PMT-based O-mannosylation is an evolutionarily conserved and vital process, key for cell wall integrity and protein quality control in fungi. PMTs are divided into three subfamilies (PMT1, PMT2, and PMT4) and form functional dimers either within or across subfamilies (Akasaka-Manya et al., 2006; Girrbach and Strahl, 2003). In these structures each subunit has 11 transmembrane helices (TMHs) and two large hydrophilic loops oriented towards the ER lumen (LL): loop LL1 between TMH1 and 2 harboring a catalytic DE motif, and loop LL4 between TMH7 and 8, encompassing a so-called MIR domain, whose function remains unknown. MIR domains have a β-trefoil fold consisting of six β-hairpins arranged within a pseudo-threefold symmetry.

The high resolution of the Pmt2-MIR (1.6 Å) and Pmt3-MIR (1.9 Å) structures allowed for a detailed analysis of the respective structural properties and ligand interactions. Amino acid ranges for Pmt2-MIR are 339–401 (MIRm1), 402–466 (MIRm2) and 467–532 (MIRm3). In order to understand the role of PMT-MIR domains in protein O-mannosylation, we analyzed the Pmt2-MIR structure for specific surface properties. On the protein surface two regions reveal high sequence conservation, in the following denoted as sites α and β (residue ranges see Figure 2) in accordance with general CBM terminology. For Pmt2, H362 and H364 are fixed in a defined orientation by a complex hydrogen-bonding pattern within the strictly conserved site α in the interface between MIRm1 and MIRm3. MIRm1 site α, which is directly adjacent to the conserved L361 of the core, is completed by residues Y380, D384, N386, F504, and Q506 forming the wall of the cavity. An almost identical arrangement is found for Pmt2-MIR site β in the MIRm1-MIRm2 interface. Both cavities are filled by ligands present in the crystallization solvent (glycerol in site α [also in Pmt3] and sulfate in site β). Although Pmt2-MIR displays a pseudo-threefold symmetry typical for the β-trefoil fold classified as Type C CBMs, the analogous site γ (the third binding site present in β-trefoils) is not present in MIRm3. However, on the surface of the β11-β12 loop a two-residue insertion is present, which is specific to the PMT2 family (including Pmt2, Pmt3, and Pmt6) and human POMTs. This loop forms a surface exposed ligand-binding site in Pmt2-MIR, from now on defined as PMT2 family-specific site δ. The three residues form a trident that has picked another glycerol ligand from the solvent via hydrogen-bonding to the arginine side chain and to the backbone amides within site δ.

> MKHHHHHHPMGLEVLFQGPPRDIALGSSVVSIKNQALGGSLLHSHIQTYPDGSNQQQVTCYGYKDANNEWFFNRERGLPSWSENETDIEYLKPGTSYRLVHKSTGRNLHTHPVAAPVSKTQWEVSGYGDNVVGDNKDNWVIEIMDQRGDEDPEKLHTLTTSFRIKNLEMGCYLAQTGNSLPEWGFRQQEVVCMKNPFKRDKRTWWNIETHENER> MYVRISGRIRLNAHSLNAQGGGGTNYIEITKTKVTVRTENGWTVVEVPAITGNMLKHWHFVGFVDYFKTTPYGVNLTERALRYNGTRFGQGETTATKANGATVQLNDEATIIKELADADVHGFLAPKTGRRRVSLVKASFILPTEDFIKEVEGERLITAIKHNRVDVDEKGAIGSSKEGTAQMLFSREYATGLYGFSIVLDLGLVGIPQGLPVKFEENQPRPNIVIDPNERKARIESAL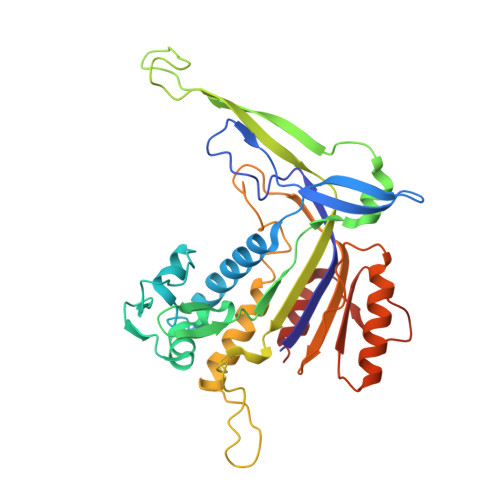KALIPMLSGYIGANLARSFPVFKVEELVAIASEGPIPALVHGFYEDYIEANRSIIKNARALGFNIEVFTYNVDLGEDIEATKVSSVEELVANLVKMV>[5x]GHMEKLKEFRGIKEHLGVFREAVKDAERIGFAGVPGVCTPFAQLFAYAVRDKDNIFIPNTDFSKARKLEVTEYGVELGEISPGNVDVLVLLGGLSMPGIGSDIEDV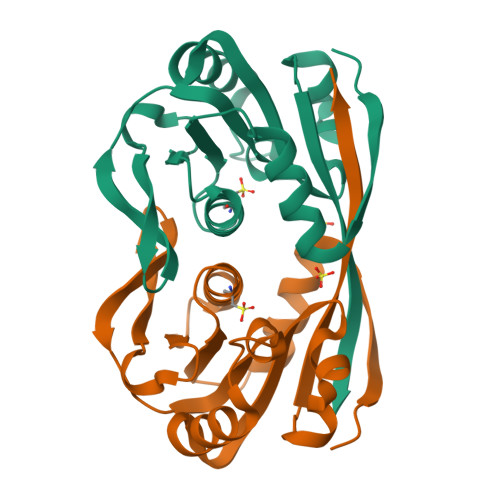KKLVEDALEEGGELMGLCYMDMFARAGWYELLDFDCVINADIDGYVLRGGS>GAMGSMNLLIMGLPGAGKGTQAAKIVEQFHVAHISTGDMFRAAMANQTEMGVLAKSYIDKGELVPDEVTNGIVKERLSQDDIKETGFLLDGYPRTIEQAHALDKTLAELGIELEGIINIEVNPDSLLERLSGRIIHRVTGETFHKVFNPPVDYKEEDYYQREDDKPETVKRRLDVNIAQGEPIIAHYRAKGLVHDIEGNQDINDVFSDIEKVLTNLK[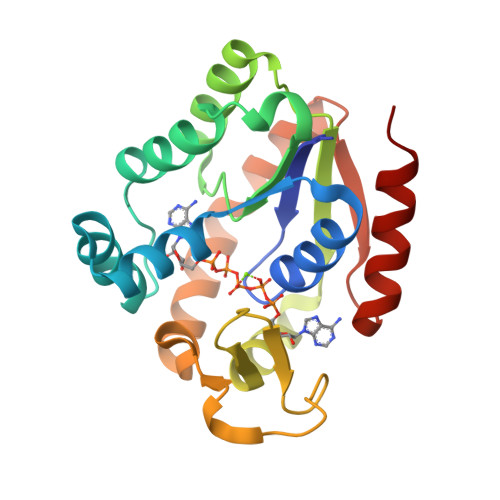2x]Protein stability can be fine‐tuned by modifying different structural features such as hydrogen‐bond networks, salt bridges, hydrophobic cores, or disulfide bridges. Among these, stabilization by salt bridges is a major challenge in protein design and engineering since their stabilizing effects show a high dependence on the structural environment in the protein, and therefore are difficult to predict and model. In this work, we explore the effects on structure and stability of an introduced salt bridge cluster in the context of three different de novo TIM barrels. The results show that despite the similarities in protein fold, the salt bridge clusters differently influence the structural and stability properties of the de novo TIM barrel variants depending on the structural background where they are introduced.

The salt bridge variants exhibit similar thermostability in comparison with their parental designs but important differences in the conformational stability at 25°C can be observed such as a highly stabilizing effect for two of the proteins but a destabilizing effect to the third. Analysis of the formed geometries of the salt bridge cluster in the crystal structures show either highly ordered salt bridge clusters or only single salt bridges. Rosetta modeling of the salt bridge clusters results in a good prediction of the tendency on stability changes but not the geometries observed in the three‐dimensional structures.

>MDKDEAWKQVEILRRLGAKRIAYRSDDWRDLQEALKKGADILIVDATDKDEAWKQVEILRRLGAKEIAYRSDDWRDLQEALKKGADILIVDATDKDEAWKQVEILRRLGAKRIAYRSDDWRDLQEALKKGADILIVDATDKDEAWKQVEILRRLGAKEIAYRSDDWRDLQEALKKGADILIVDATGLEHHHHHH[2x]> MAGIAMKLAKDREAAEGLGSHERAIKYLNQDYETLRNECLEAGALFQDPSFPALPSSLGFKELGPYSSKTRGIEWKRPTEICADPQFIIGGATRTDICQGALGDSWLLAAIASLTLNEEILARVVPLDQSFQENYAGIFHFQFWQYGEWVEVVVDDRLPTKDGELLFVHSAEGSE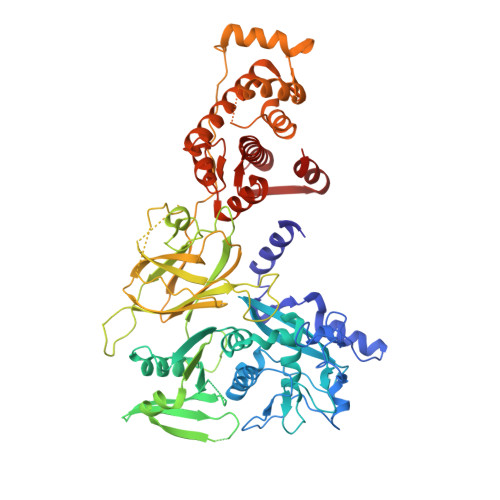FWSALLEKAYAKINGCYEALSGGATTEGFEDFTGGIAEWYELRKPPPNLFKIIQKALEKGSLLGCSIDITSAADSEAVTYQKLVKGHAYSVTGAEEVESSGSLQKLIRIRNPWGQVEWTGKWNDNCPSWNTVDPEVRANLTERQEDGEFWMSFSDFLRHYSRLEICNLTPDTLTCDSYKKWKLTKMDGNWRRGSTAGGCRNYPNTFWMNPQYLIKLEEEDEDDEDGERGCTFLVGLIQKHRRRQRKMGEDMHTIGFGIYEVPEELTGQTNIHLSKNFFLTTRARERSDTFINLREVLNRFKLPPGEYVLVPSTFEPHKNGDFCIRVFSEKKADYQTVDDEIEANIEEIEANEEDIGDGFRRLFAQLAGEDAEISAFELQTILRRVLAKREDIKSDGFSIETCKIMVDMLDEDGSGKLGLKEFYILWTKIQKYQKIYREIDVDRSGTMNSYEMRKALEEAGFKLPCQLHQVIVARFADDELIIDFDNFVRCLVRLEILFKIFKQLDPENTGTIQLDLISWLSFSVL> MANTKYNEEFLLYLAGFVDSDGSIIAQIKPRQSNKFKHQLSLTFAVTQKTQRRWFLDKLVDEIGVGYVYDSGSVSDYRLSEIKPLHNFLTQLQPFLKLKQKQANLVLKIIEQLPSAKESPDKFLEVCTWVDQIAALNDSKTRKTTSETVRAVLDS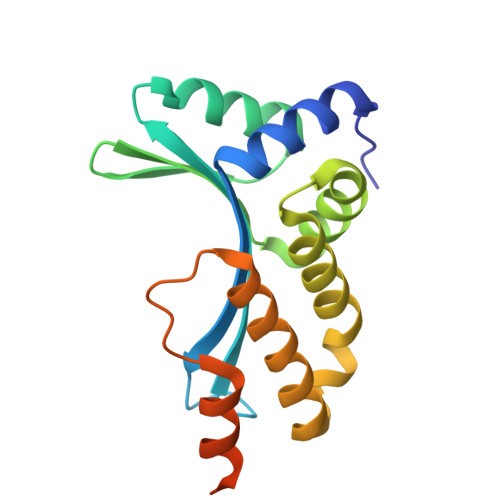LSEKKKSSPAADHHHHHH5-methyl-~{N}-[[(2~{S})-oxolan-2-yl]methyl]-1,2-thiazole-3-carboxamide 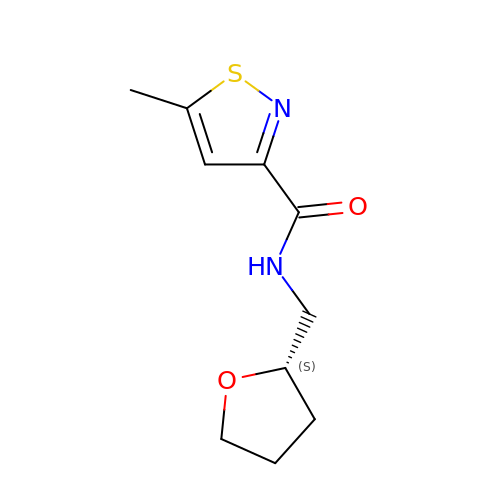| C10 H14 N2 O2 S | PYHOSVJXCWPVCG-QMMMGPOBSA-N>XEKNALLRYLLDKDX[13x]

Nuclear hormone receptors are cytoplasm-based transcription factors that bind a ligand, translate to the nucleus and initiate gene transcription in complex with a co-activator such as TIF2 (transcriptional intermediary factor 2). For structural studies the co-activator is usually mimicked by a peptide of circa 13 residues, which for the largest part forms an α-helix when bound to the receptor. HPLC analysis of the crystals revealed the absence of the receptor and indicated that only the co-activator peptide was present.

A beautiful but unanticipated structure was obtained that forms superhelices with left-handed twist throughout the crystal, stabilized by ligand interactions. Placement of the 13 TIF2 helices into closest proximity revealed their arrangement as a superhelix of outer diameter 42 × 46 Å. The helices are not arranged parallel to each other but are organized in pairs which point their C-termini towards each other and the N-termini are located on the surface of the superhelix. The strong left-handed twist in TIF2 therefore comes as an exception, being the only all α-helical motif that assembles into such a superhelix. In contrast, when crystallized alone the TIF2 peptide forms an α-helix over its entire length less the C-terminal aspartyl amide, but including the N-terminal acetyl group. The conformation of TIF2 that is present in the superhelix would clash with residues from GR, explaining why the helix of the co-activator peptide must be shorter when bound to the receptor. In addition, non-proteinaceous electron density identified a molecule that is wedged between two adjacent TIF2 helices and that mediates contact between them by means of hydrogen bonds and van der Waals interactions. From the SHELXE density alone it was clear that the ligand is a steroid, which was unanticipated but is easily explained by the buffer component CHAPS, an amide of cholic acid. Cholic acid is a convex molecule that fits into a concave surface patch lined by the methylene groups of Glu1, the side chains of Ala4 and Leu5, and the aromatic face of the Tyr8 side chain. A hydroxyl group of the steroid binds to the carbonyl group of the Asn3 carboxamide, and the carboxylate of cholic acid engages in a (possibly charged) hydrogen bond with the guanidinium group of Arg7.>ALRNQIEQFLGAIMQFAENKHEILLGECESNVKLTSTQEHILMILAAEVSTNARIAEQLKISPAAVTKALKKLQEQELIKSSRATNDERVVLWSLTEKAIPV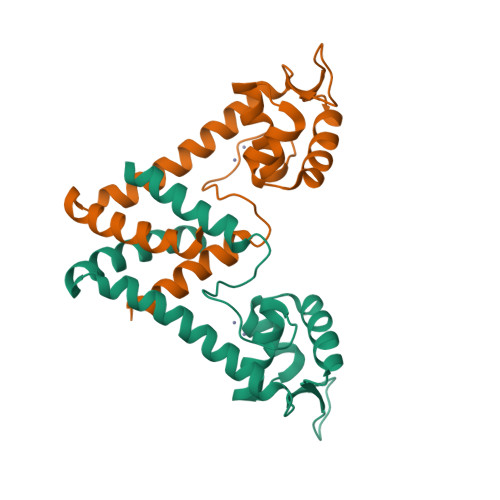AKEHAAHHEKTLSTYQELGDKFTDEEQKVISQFLSVLTEEFR[8x]~{N}2,~{N}6,9-trimethylpurine-2,6-diamine | C8 H12 N6 | 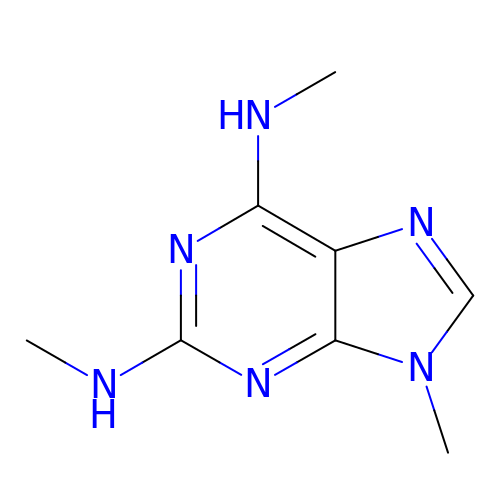YFZMXDSHFHHAQH-UHFFFAOYSA-N> MGAEKKLFLKALKEKFEEDPKEKYTKFYVF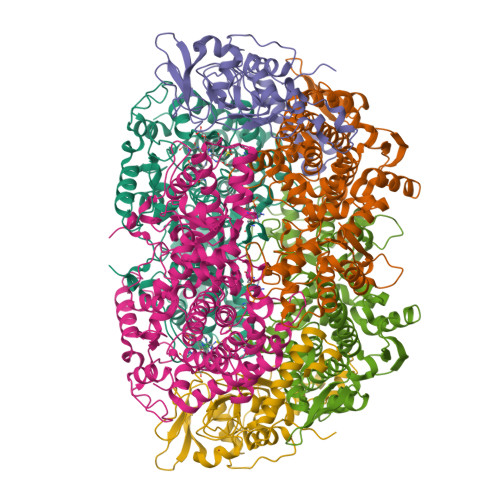GGWRQSARKREFVEAAEKLAEKRGGIPFYNPDIGVPLGQRKLMPYKLSGTDYIVEGDDLHFMNNAAMQQFWDDIRRTVIVGMDTAHAVLEKRLGVEVTPETINEYMETINHALPGGAVVQEHMVEVHPALAWDCYAKIFTGDDELADEIDKKFLIDINKLFPEEQAEQLKAAIGKRTYQVSRVPTLVGRVCDGGTIARWSAMQIGMSFITAYKLCAGEAAIADFSYAAKHADVIQMGTLLPARRARGPNEPGGIPFGILADVVQTTRVSDDPVEQSLEVVASGAMLYDQIWLGSYMSGGVGFTQYATASYTDDILDDFSYYGYDYVEKKYGICGAKPTMDVVEDIATEVTLYALECYDEFPALLEDHFGGSQRAAVAAAASGISVCMATGNSNAGLNGWYLSQILHKEYHSRLGFYGYDLQDQCGASNSLSIRNDESSPLELRGPNYPNYAMNVGHQGEYAGITQAAHSARKDAFALNPLIKVAFADPSLVFDFSHPRKEFARGALREFEPAGERDPIIPAH;> MVKYEDKICLYNAKGELVEENVPLEAISPLYNPTIQKLVKDIKRTVAVNLAGIENALKTGAVGGKACVIPGRTLDLPIVENAETIMEYVDKLLRISPDDDTSVKLINDGKQMAVQLPSKRLEVAAEYSISMLNTAMALKEAIIKTFDVDMFDAPMVHAAILGRYPQVPDYMGANIASLLGAPTNLEGLGYALRNIMVNHYVATTKKNIMNAVAFASIMEQTAMFEMGDAIGSFERLHLLGLAYQGLNADNLVIDLVKANGKNGTVGTVVASIVERALEDGVITEDKKMPSGFVLYKPVDVAKWNAYAAAGLVAAVIVNCGAARAAQNVASTILYYNDIIEYETGLPGVDFGRAEGTAVGFSFFSHSIYGGGGPGIFNGNHIVTRHSKGFAIPPVCAAMCVDAGTQMFSPEKTSALVGAVFSAIDEFREPLKYVIDGALAVKDKI;> MAYKPQFYPGETKIAQNRRNHMNPEVELEKLREIPDEDVVKIMGHRQPGEDYKTIHPPLEEMDLPDDYVRDLVEPINGAKEGHRIRYIQFADSMYFAPAQPYDRARTYMWRFRGVDTGTLSGRQVIEMRESDLEALSKNFLIDTAFFDPARCGIRGATVHGHSLRLDENGLMFDALQRYVYDEKTGHVVYVKDQVGRPLDEPVDVGELLPEEKLREITTIYRKDGVPMREDKELLTIVKRIHRARTLGGFCPTEDTFKQL>[4x]HHH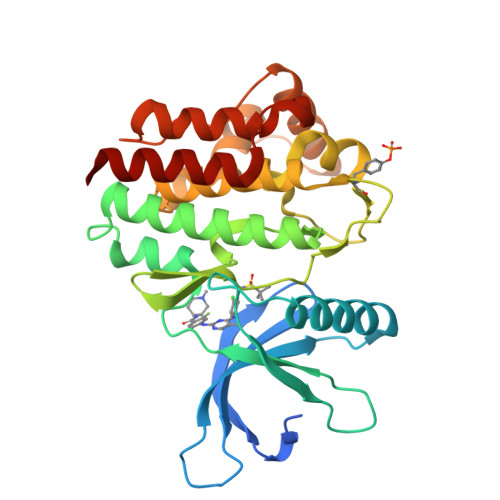HHHHHENLYFQGDPTQFEERHLKFLQQLGKGNFGSVEMCRYDPLQDNTGEVVAVKKLQHSTEEHLRDFEREIEILKSLQHDNIVKYKGVCYSAGRRNLKLIMEYLPYGSLRDYLQKHKERIDHIKLLQYTSQICKGMEYLGTKRYIHRDLATRNILVENENRVKIGDFGLTKVLPQDKEYYKVKEPGESPIFWYAPESLTESKFSVASDVWSFGVVLYELFTYIEKSKSPPAEFMRMIGNDKQGQMIVFHLIELLKNNGRLPRPDGCPDEIYMIMTECWNNNVNQRPSFRDLALRVDQIRDNMAG3-[8-({4-[ethyl(2-hydroxyethyl)amino]phenyl}amino)imidazo[1,2-a]pyrazin-5-yl]phenol | 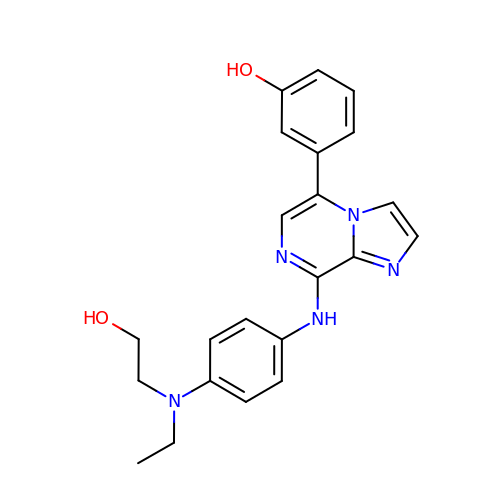C22 H23 N5 O2 | HNXXZSFGRGLZTI-UHFFFAOYSA-N>[5x]GSHMA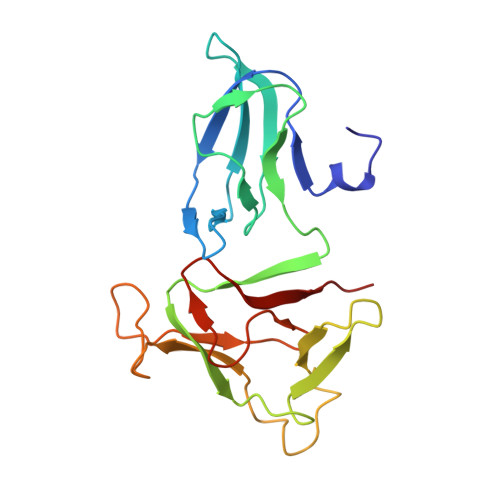AAESSIQVKNKGSIKLSNVKSVVNSSGKLVITSRNTELKLIDEFGRTKESYKVPYGAVLAKGDGEQVAGGETVANWDPHTMPVITEVSGFVRFTDMIDGQTITRQTDELTGLSSLVVLDSAERTAGGKDLRPALKIVDAQGNDVLIPGTDMPAQYFLPGKAIVQLEDGVQISSGDTLARIPQESG> MAEELVLERCDLELETNGRDHHTADLCREKLVVRRGQPFWLTLHFEGRNYQASVDSLTFSVVTGPAPSQEAGTKARFPLRDAVEEGDWTATVVDQQDCTLSLQLTTPANAPIGLYRLSLEASTGYQGSSFVLGHFILLFNAWCPADAVYLDSEEERQEYVLTQQGFIYQGSAKFIKNIPWNFGQFQDGILDICLILLDVNPKFLKNAGRDCSRRSSPVYVGRVGSGMVNCNDDQGVLLGRWDNNYGDGVSPMSWIGSVDILRRWKNHGCQRVKYGQCWVFAAVACTVLRCLGIPTRVVTNYNSAHDQNSNLLIEYFRNEFGEIQGDKSEMIWNFHCWVESWMTRPDLQPGYEGWQALDPTPQEKSEGTYCCGPVPVRAIKEGDLSTKYDAPFVFAEVNADVVDWIQQDDGSVHKSINRSLIVGLKISTKSVGRDEREDITHTYKYPEGSSEEREAFTRANHLNKLAEKEETGMAMRIRVGQSMNMGSDFDVFAHITNNTAEEYVCRLLLCARTVSYNGILGPECGTKYLLNLTLEPFSEKSVPLCILYEKYRDCLTESNLIKVRALLVEPVINSYLLAERD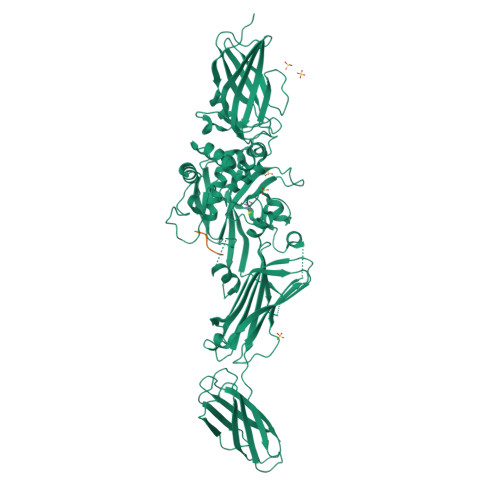LYLENPEIKIRILGEPKQKRKLVAEVSLQNPLPVALEGCTFTVEGAGLTEEQKTVEIPDPVEAGEEVKVRMDLVPLHMGLHKLVVNFESDKLKAVKGFRNVIIGPA> MQNGYTYEDYQDTAKWLLSHTEQRPQVAVICGSGLGGLVNKLTQAQTFDYSEIPNFPESTVPGHAGRLVFGILNGRACVMMQGRFHMYEGYPFWKVTFPVRVFRLLGVETLVVTNAAGGLN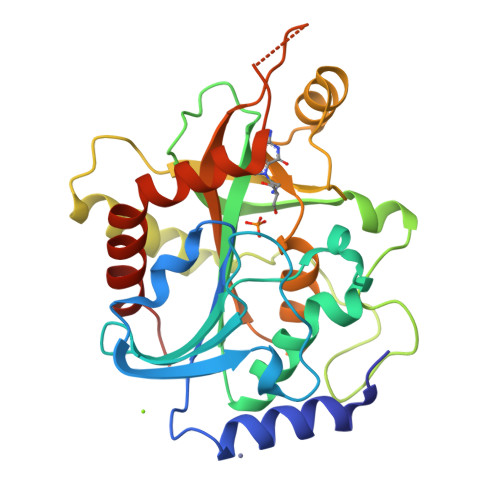PNFEVGDIMLIRDHINLPGFSGQNPLRGPNEERFGVRFPAMSDAYDRDMRQKAHSTWKQMGEQRELQEGTYVMLGGPNFETVAECRLLRNLGADAVGMSTVPEVIVARHCGLRVFGFSLITNKVIMDTESQGKANHEEVLEAGKQAAQKLEQFVSLLMASIPVSGHTG>MVRPSQSMYDRHLTIFSPDGNLYQIEYAIKAVKNTNITSVGVKGENCAVIISQKKMATQYISQDKLLDYNNITNIYNITDEIGCSMVGMPGDCLSMVYKARSEASEFLYSNGYNVNAETLCRNICDKIQVYTQHAYMRLHACSGMIIGIDENNKPELFKFDPSGFCAGYRACVIGNKEQESISVLERLLEKRKKKIQQETIDEDIRNTTILAIEALQTILAFDLKASEIEVAIVSTKNRNFTQISEKEIDNYLTYIAERD[2x];>[2x]MADGEYSFSLTTFSPTGKLVQIEYALNRVSSSSPALGIRAKNGVIIATEKKSPNELIEENSIFKIQQISEHIGIVYAGMPGDFRVLLKRARKEAIRYSLQYGSEILVKELVKIIASIVQEFTQTGGVRPFGLSLLICGVDVYGYHLYQIDPSGCYFNWMATCVGKDYQNNMSFLEKRYNKDIEIEDAIHTAILTLKESYEGVLNEKNIEIGVAYDNKPFKILTQNEIKDYLIEIE;>MARRYDSRTTTFSPEGRLYQVEYALEAINNASITIGLITKDGVILGADKVFISKLIDKANNYEKIYKIDKHIFCGVAGLNADANILINQSRLYAQRYLYNYNEVQPVSQLVVQICDIKQSYTQYGGLRPYGVSFLIGGYDTKDGYQLYHTDPSGNYSGWFATAIGTNNLTASSVLKQEWKNDMTLEEGLLLALKTLAKSTDTEIPKSEKIELAYLTNKDGEVYQKYLTEKEIEELIKLYTQKYIKE[2x];>MSYDRAITVFSPDGHLLQVEHALEAVKKGGCAVAIKSSNFAVLAVEKKNIPKLQNPKTTEKLIKLDEHNCLAF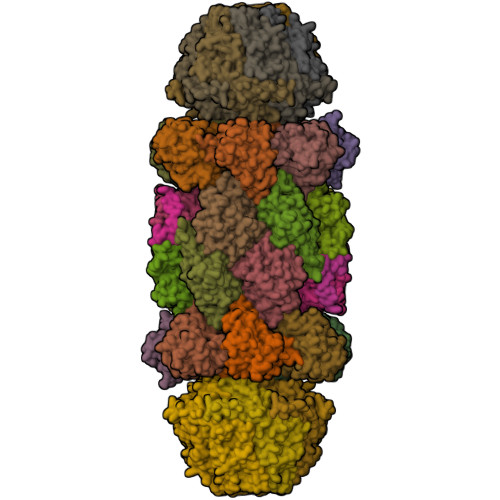AGLNADARVLVNKTRLECQRYYLNMDEPAPVDYIAKYVAKVQQKFTHRGGVRPFGIATLIAGFKNNKEICIYQTEPSGIYAAWKAQAIGKNAKIVQEFLEKNYQENMEQKDCIFLALKAIFEVVELSSKNVEVALLTEKDLTFIEEQEINSMVELIDQERTKNNEQNE[2x];>[2x]MFSTRSEYDRGVNTFSPEGRLFQVEYALGAIKLGSTAVGICVNDGVILASERRISSTLIEKDSVEKLLSIDDHIGCAMSGLMADARTLIDYARVECNHYKFIYNENINIKSCVELISELALDFSNLSDSKRKKIMSRPFGVALLIGGVDKNGPCLWYTEPSGTNTRFSAASIGSAQEGAELLLQENYKKDMTFEQAEILALTVLRQVMEDKLSTSNVEICAIKKSDQTFYKYNTDDISRIIDVLPSPVYPTIDMTA;>MYRNLYDTDNIIYSPEGRLYQVEYASEAIKQGTCAVAIKSKDYVVVSGLKKCISKLSFPQEKIFKIDDYIGISMSGITSDAKVLTKFMQNECLSHKFLYNENINIESLVRSVADKYQKNTQKSSKRAFGVGLMIAAYHNEPCIFETRPNGSYFEYDALSFGARSHASKTYLEKNLHLFEECSLEELILHCLKALKCSLSSESELTISNTALAVVGKNHPWQEISSLQLEEYLSKVKMDAEQEQVEENVQNEANE[2x];>MAGLSAGYDLSVSTFSPDGRLYQVEYIYKSINNNNTALCLECKDGIICCCINSNMDKNKMIKKNSYNRIYHVNNNIIITYSGFDGDARNIIDRARSEANTYYYNFHTNIPLHILVNRISLYIHAYTLYWHMRPFAASIIISSFNEKDKGDIYCIEPNGACYKYSGIVIGKNKEMFKTEIEKKDYKDINVRDAIEDIYKFILTSDDHMNKNNLQNLVNFSWICKESSYEFQNIHEEILTPALNKAVEYIEKLN[2x];>TTIIGIIYDNGVMLACDSRTSSGTFISNKCSRKINRINENLYVCRSGASAHSQKIIEIIKHYCVSMKNENRKKGRFHEGETIYDETTYDEEIDIDSINYLDYNNNNDNNLVTKNKYFYEDKFNDYNPLVENVAHITKKIIYTNNNFLSCALIFGGYDKIKKQQLYAVNLNGSIIEKHDFAVSGSGSIYIQSYLQDKYKKFMTKKECFNLILNCVKYAMHNDNSSGGLIRIVNITKSFVEEFTVVNTQMNFQY[2x];>[2x]TTICGLVCQNAVILGADTRATEGPIVADKNCSKLHYISKNIWCAGAGVAGDLEHTTLWLQHNVELHRLNTNTQPRVSMCVSRLTQELFKYQGYKVCAIVLGGVDVNGPQLYGIHPHGSSCLLPFTALGSGSLNAMAVLEAKYRDNMTIEEGKNLVCEAICAGIFNDLGSGGNVDICVITKDSYQHIRPYKEPNMRLYHLPHPTIYPKGTTPILSEKIEYIKKFISVEDA;>[2x]MGSIYNYNGGCVLGMSGSNCVAIACDLRLGANTFTTVSTKFSKIFKMNNNVYVGLSGLATDIQTLYEILRYRVNLYEVRQDAEMDVECFANMLSSILYSNRFSPYFVNPIVVGFKLKHYVDEEGEKKVNYEPYLTAYDLIGAKCETRDFVVNGVTSEQLFGMCESLYVKDQDENGLFETISQCLLSALDRDCISGWGAEVLVLTPEKIIKKKLKARMD;>MDTLIGLRGNNFVVLAADTYSINSIIKLKNDDNTKFYDIHGNKCLLLGGSIGDRLQFGEFIRKNVHLYQYQNNTDMFVKSFAFFTRKNLAYYLRRNPFEVNCLIAGYDKKDGYQLYWCDYLSNMDSVNKGAHGYGAYLVSAILDKYYHENLTVDEALDIFKLCFEELKKRFLLTQINYELRIMYDNKVETQYVTV[2x];>[2x]TTTLAFKFKDGIIVAVDSRASMGSFISSQNVEKIIEINKNILGTMAGGAADCLYWEKYLGKIIKIYELRNNEKISVRAASTILSNILYQYKGYGLCCGIILSGYDHTGFNMFYVDDSGKKVEGNLFSCGSGSTYAYSILDSAYDYNLNLDQAVELARNAIYHATFRDGGSGGKVRVFHIHKNGYDKIIEGEDVFDLHYHYTNPEQKDQYVM;>[2x]MDLILYNDNLTEKKTEKENVIEHGRGFKRWYPYIDNGGTVIGLTGKDYVILAADTRLSLSYSIYTRFCPKISKLTDKCIIGSSGMQSDIKTLHSLLQKKIQLFVLEHSHYPDIHVIARLLCVILYSRRFFPYYAFNILAGVDENNKGVLYNYDSVGSYCEATHSCVGSGSQLILPILDNRVEQKNQLIKNTNFNLGDDINFVKDAITSATERDIYTGDKTLIYVIDKMGINVNTLDLKQD;>MTLGPVVTGTSVIAIKYKHGIMIAADRKASYGSYAKFQNVERIFKINNKTVMGFSGELADAQYLHELLTRKNINNLSEKKRKEDMYTPQHYHSYVSRVFYVRKNRIDPLFNNIIIAGINSQKYDNNDDNVLLYTNKNNDDEQNEYKNNEEYKEIHKDDLYIGFVDMHGTNFCDDYITTGYARYFALTLLRDHYKDNMTEEEARILINECLRILYFRDATSSNFIQIVKVTSKGVEYEEPYILPCVLNSADYVYPSTLLPPAGCMW[2x];>MEAYLNKIDKIEPSDQKIKEEYNKFKYDITKQAIESLRERIPKRIIFFNNLVNVNSEPGSILNVNDLDGVSYKYKINKIEENVRKKHKGNNSSDFDEREKKKDSLDGHVKHFSNNEDSKLIIDDKVLYTHYVPSHKQIYLELEKIKTYASELIEIIGNIKLWIQLNVPRIEDGNNFGVGIQEEAIQELARVEESAFNLYDAIVKYYMERAKISTKVLKYPNVSDYQEAVRELDEKEWIHIKITIVDMRNNYIMLYDLLYKNWEKVVKPKNEDAHHRMTF[14x]4-(2-carboxyphenyl)carbonyl-2-nitro-benzoic 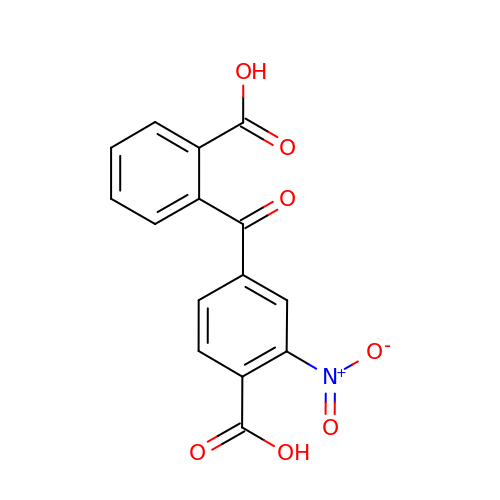acid | C15 H9 N O7 | WDYTXQOHLZPDFS-UHFFFAOYSA-N>[2x]AEGGFLEDAKTDLVLRNYYFNRDFRDHDAGKSLVDEWAQGFILKFSSGYTPGTVGVGLDAIGLFGVKLNSGRGTSNSELLPLHDDGRAADNYGRVGVAAKLRVSASELKIGEMLPDIPLLRY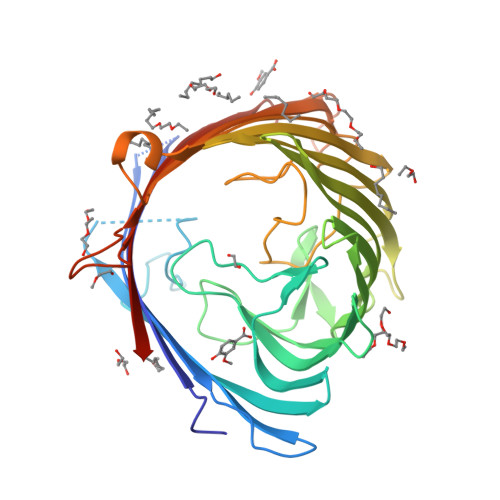DDGRLLPQTFRGFAVVSRELPGLALQAGRFDAVSLRNSADMQDLSAWSAPTQKSDGFNYAGAEYRFNRERTQLGLWHGQLEDVYRQSYANLLHKQRVGDWTLGANLGLFVDRDDGAARAGEIDSHTVYGLFSAGIGLHTFYLGLQKVGGDSGWQSVYGSSGRSMGNDMFNGNFTNADERSWQVRYDYDFVGLGWPGLIGMVRYGHGSNATTKAGSGGKEWERDVELGYTVQSGPLARLNVRLNHASNRRSFNSDFDQTRLVVSYPLSWGGHHHHHH> MADVKLHGSWVSPFNYRVIWALKLKGVEFEHIVEDLTNKSELLLKYNPVYKKIPVLVHGGKPIAESLVILEYIEETWPENPLLPTDPYERAMARFWIQYGATKTAAFGALFRASGEELEKAAKEVVEVLRVLEEQGLGDKKFFGGDSINLVDISFGLFTCWL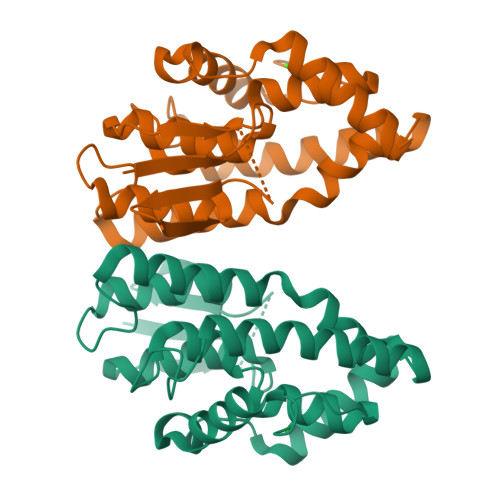EAIEEAAGVKVLEPSTLPRLHAWAQNFIEVPLIKENIPDYDKLLLHMKGVREKMMNK>[4x]MAKDIGINSDPNSSSVDKLMKSSGVSNPTYTLVWKVWILAVTLYYAIRIPLTLVFPSLFSPLLPLDILASLALIADIPLDLAFESRRTSGRKPTLLAPSRLPDLLAALPLDLLVFALHLPSPLSLLSLVRLLKLISVQRSATRILSYRINPALLRLLSLVGFILLAAHGIACGWMSLQPPSENPAGTRYLSAFYWTITTLTTIGYGDITPSTPTQT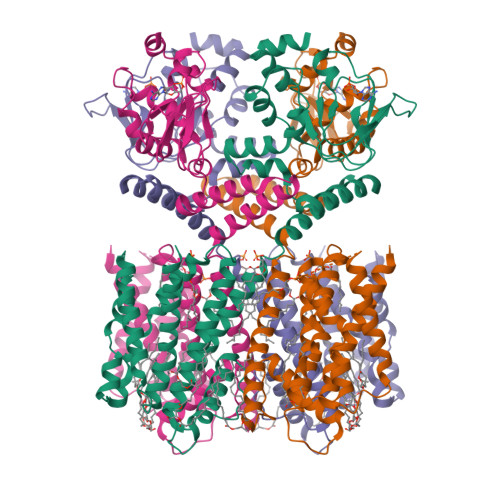VYTIVIELLGAAMYGLVIGNIASLVSKLDAAKLLHRERVERVTAFLSYKRISPELQRRIIEYFDYLWETRRGYEEREVLKELPHPLRLAVAMEIHGDVIEKVALFKGAGEEFIRDIILHLEPVIYGPGEYIIRAGEMGSDVYFINRGSVEVLSADEKTRYAILSEGQFFGEMALILRAPRTATVRARAFCDLYRLDKETFDRILSRYPEIAAQIQELAVRRKELESSGLVPRGSVKHHHH>MNHKVHHHHHHLQENLYFQGMEMEAPLIVIVPSPGMGHLIPLVEFAKVLVSRFHFSVSLLLPTTAQPTKAQTTLLNSLPSSVSHNFLPTVDPAHLPDGVAHEVTISLTHAHSLSSIRAALGSLAQQAQVVALITDLFGTGLYTVARDLGIPPYLYFTSTAMCLLFLFHLPKLDETVSCEYRDMPEPLVLPGCVPLHGKDFVDPAQDRQDQAYHVLLDHVKRYVLAEGIFVNTFVDLEPGAIKTLQTEDPNVPPVYPVGPIIQSGLDDDSHGSDCLKWLDRQPSGSVLFVSFGSGGTLSNEQLNELAIGLEISGHRFLWVVRSPNDHSSFGSFFSTQSQDDPFGFLPTGFVDRIKDRGLLVPSWAPQIKV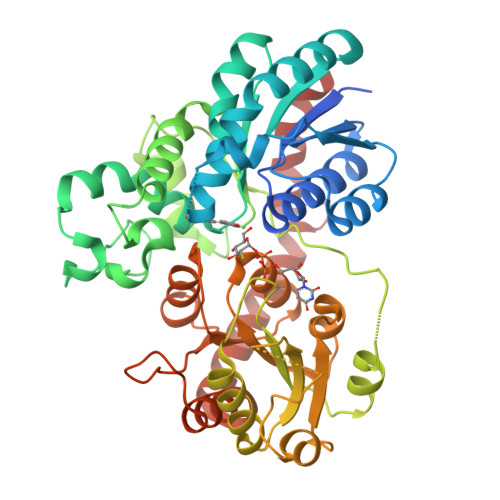LSHGSTGGFLTHCGWNSTLESIVNGVPLIVWPLYAEQRMNAVMLNQGLKVALRPNASQRGLVEADEIARVVKELMDGDEGKKARYKMRELSDSAKRVTSENGESTKLLSEVASKWSQCKS[3x]> MDYQEYQQFLARINTARDACVAKDIDVDLLMARKDYFGRELCKSLNIEYRNDVPFIDIILDIRPEVDPLTIDAPHITPDNYLYINNVLYIIDYKVSVSNESSVITYDKYYELTRDISDRLSIPIEIVIIRIDPVSRDLHINSDRFKELYPTIVVDINFNQFFDLKQLLYEKFGDDEEFLLKVAHGDFTLTAPWCKTGCPEFWKHPIYKEFKMSMPVPERRLFEESVKFNAYESERWNTNLVKIREYTKKDYSEHISKSAKNIFLASGFYKQPNKNEISEGWTLMVERVQDQREISKSLHDQKPSIHFIWGAHNPGNSNNATFKLILLSKSLQSIKGISTYTEAFKSLGKMMDIGDKAIEYEEFCMSLKSKARSSWKQIMNKKLEPKQINNALVLWEQQFMINNDLIDKSEKLKLFKNFCGIGKHKQFKNKMLEDLEVSKPKILDFDDANMYLASLTMMEQSKKILSKSNGLKPDNFILNEFGSRIKDANKETYDNMHKIFETGYWQCISDFSTLMKNILSVSQYNRHNTFRIAMCANNNVFAIVFPSADIKTKKATVVYSIIVLHKEEENIFNPGCLHGTFKCMNGYISISRAIRLDKERCQRIVSSPGLFLTTCLLFKHDNPTLVMSDIMNFSIYTSLSITKSVLSLTEPARYMIMNSLAISSNVKDYIAEKFSPYTKTLFSVYMTRLIKNACFDAYDQRQRVQLRDIYLSDYDITQKGIKDNRELTSIWFPGSVTLKEYLTQIYLPFYFNAKGLHEKHHVMVDLAKTILEIECEQRENIKEIWSTNCTKQTVNLKILIHSLCKNLLADTSRHNHLRNRIENRNNFRRSITTISTFTSSKSCLKIGDFRKEKELQSVKQKKILEVQSRKMRLANPMFVTDEQVCLEVGHCNYEMLRNAMPNYTDYISTKVFDRLYELLDKKVLTDKPVIEQIMDMMIDHKKFYFTFFNKGQKTSKDREIFVGEYEAKMCMYAVERIA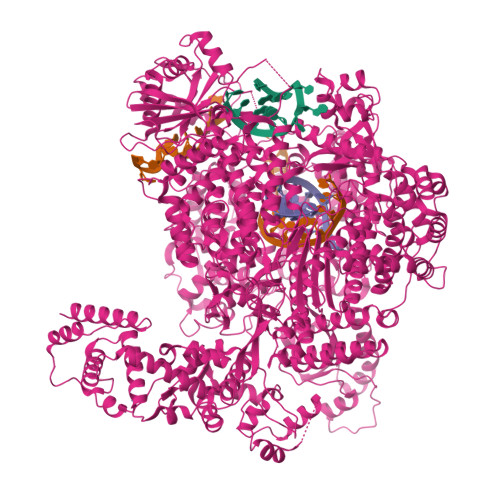KERCKLNPDEMISEPGDGKLKVLEQKSEQEIRFLVETTRQKNREIDEAIEALATEGSGWSHPQFEKGSGYESNLGKIEKLSLGKAKGLKMEINADMSKWSAQDVFYKYFWLIALDPILYPQEKERILYFMCNYMDKELILPDELLFNLLDQKVAYQNDIIATMTNQLNSNTVLIKRNWLQGNFNYTSSYVHSCAMSVYKEILKEAITLLDGSILVNSLVHSDDNQTSITIVQDKMENDKIIDFAMKEFERACLTFGCQANMKKTYVTNCIKEFVSLFNLYGEPFSIYGRFLLTSVGDCAYIGPYEDLASRISSAQTAIKHGCPPSLAWVSIAISHWMTSLTYNMLPGQSNDPIDYFPAENRKDIPIELNGVLDAPLSMISTVGLESGNLYFLIKLLSKYTPVMQKRESVVNQIAEVKNWKVEDLTDNEIFRLKILRYLVLDAEMDPSDIMGETSDMRGRSILTPRKFTTAGSLRKLYSFSKYQDRLSSPGGMVELFTYLLEKPELLVTKGEDMKDYMESVIFRYNSKRFKESLSIQNPAQLFIEQILFSHKPVIDFSGIRDKYINLHDSRALEKEPDILGKVTFTEAYRLLMRDLSSLELTNDDIQVIYSYIILNDPMMITIANTHILSIYGSPQRRMGMSCSTMPEFRNLKLIHHSPALVLRAYSKNNPDIQGADPTEMARDLVHLKEFVENTNLEEKMKVRIAMNEAEKGQRDIVFELKEMTRFYQVCYEYVKSTEHKIKVFILPAKSYTTTDFCSLMQGNLIKDKEWYTVHYLKQILSGGHKAIMQHNATSEQNIAFECFKLITHFADSFIDSLSRSAFLQLIIDEFSYKDVKVSKLYDIIKNGYNRTDFIPLLFRTGDLRQADLDKYDAMKSHERVTWNDWQTSRHLDMGSINLTITGYNRSITIIGEDNKLTYAELCLTRKTPENITISGRKLLGSRHGLKFENMSKIQTYPGNYYITYRKKDRHQFVYQIHSHESITRRNEEHMAIRTRIYNEITPVCVVNVAEVDGDQRILIRSLDYLNNDIFSLSRIKVGLDEFATIKKAHFSKMVSFEGPPIKTGLLDLTELMKSQDLLNLNYDNIRNSNLISFSKLICCEGSDNINDGLEFLSDDPMNFTEGEAIHSTPIFNIYYSKRGERHMTYRNAIKLLIERETKIFEEAFTFSENGFISPENLGCLEAVVSLIKLLKTNEWSTVIDKCIHICLIKNGMDHMYHSFDVPKCFMGNPITRDINWVMFREFINSLPGTDIPPWNVMTENFKKKCIALINSKFETQRDFSEFTKLMKKEGGRSNIEFD> MNGTGGAFEGGLFSPYLTTRLPGWAGVRQNVMGSTVDGRPVLPANSSTMTYATVGNSSL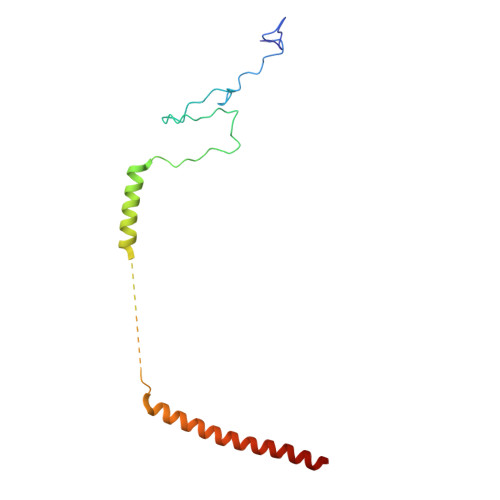DSTAAAAAAAAAMTATRLASSYMPSSGSSPSVPSSIIAEEKLLALLAELEALSRQLAALTQQVSELREQQQQQNK{(1R,2S,4R)-4-[(5-{4-[(1R)-3,4-dihydro-1H-2-benzopyran-1-yl]thiophene-2-carbonyl}pyrimidin-4-yl)amino]-2-hydroxycyclopentyl}methyl 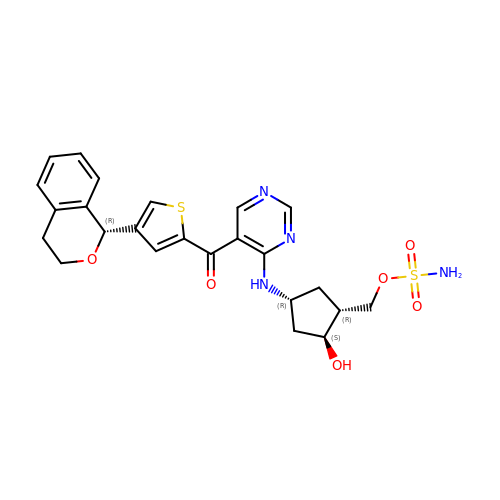sulfamate | C24 H26 N4 O6 S2 | HKKCQZRJLCIYQD-NPDZVAPOSA-N N-(3,3-dimethyl-2,3-dihydro-1H-indol-6-yl)-2-[(pyridin-4-ylmethyl)amino]pyridine-3-carboxamide 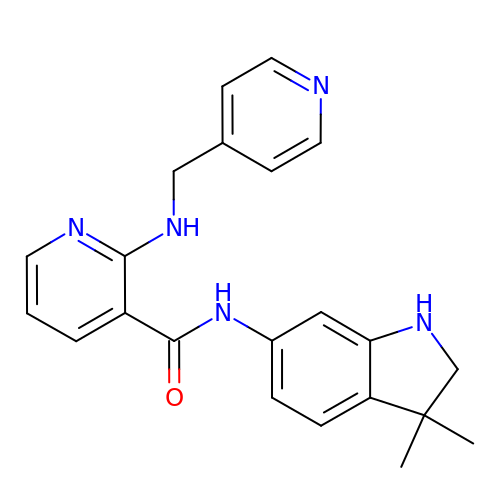| C22 H23 N5 O | RAHBGWKEPAQNFF-UHFFFAOYSA-N7-(3,5-dimethyl-1,2-oxazol-4-yl)-6-methoxy-2-methyl-N-(1-methyl-1H-indazol-3-yl)-9H-pyrimido[4,5-b]indol-4-amine 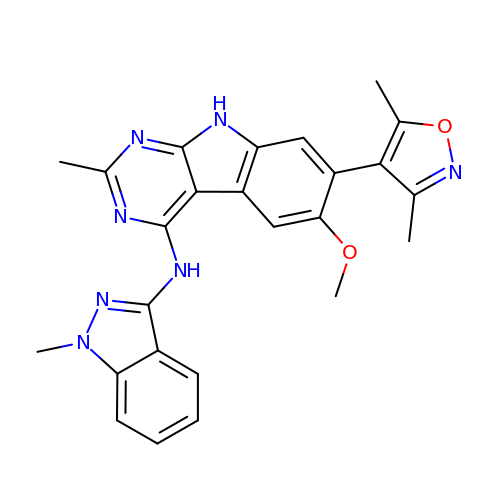| C25 H23 N7 O2 | MQUZTKXBCFOZRW-UHFFFAOYSA-N> TSWRSEATFQFTVER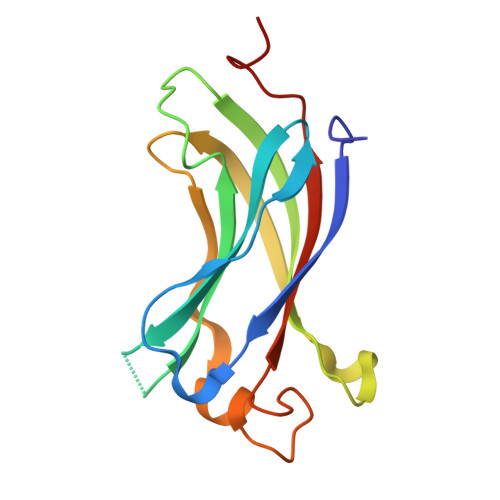FSRLSESVLSPPCFVRNLPWKIMVMPRFYPDRPHQKSVGFFLQCNAESDSTSWSCHAQAVLKIINYRDDEKSFSRRISHLFFHKENDWGFSNFMAWSEVTDPEKGFIDDDKVTFEVFVQADAPHGVAW pmcAlcohol dehydrogenases (ADHs EC 1.1.1.1) are NAD(P)H‐dependent medium‐chain oxidoreductases found in all kingdoms of life. These enzymes typically catalyse the reversible reduction of aldehydes or ketones to the corresponding alcohol. The structural motifs of ADHs are highly conserved in all known eukaryotic examples; most notably, a zinc ion involved in catalysis, a second zinc ion involved in maintaining protein structure, and the Rossmann peptide‐fold involved in cofactor binding. ADHs have been shown to catalyse many complex biochemical transformations in plant natural product biosynthesis, suggesting that their catalytic repertoire has been expanded.

For example, we recently reported the discovery of dihydroprecondylocarpine acetate synthase (DPAS), an ADH involved in vinblastine biosynthesis in the plant Catharanthus roseus and in ibogaine biosynthesis in the phylogenetically related species Tabernanthe iboga. The recently discovered DPAS reduces the substrate precondylocarpine acetate to yield an initial, unstable product, which is hypothesised to be dihydroprecondylocarpine acetate. The site of incorporation indicates DPAS catalyses the 1,4‐reduction of the α,β‐unsaturated iminium moiety and is thereby the first reported ADH with 1,4‐reduction activity. We report four crystal structures of apo‐ and substrate‐bound DPAS from two phylogenetically related species. These structures reveal, surprisingly, the loss of the catalytic zinc ion from the DPAS active site, indicating that zinc is not strictly required for reduction by ADHs. Although electron density for the structural zinc ion was clearly observed in all TiDPAS2 structures (the CrDPAS structure lacked electron density for this region), surprisingly, the substrate pocket lacked electron density at the expected site of the catalytic zinc. The lack of the catalytic zinc in DPAS is substantiated by the observation that two of the conserved catalytic zinc coordinating residues are mutated (His74Met and Cys168Ser). To investigate the catalytic mechanism of CrDPAS, we performed site directed mutagenesis of key residues involved in coordination of the catalytic zinc and the proton relay. A DPAS mutant in which the zinc ion coordinating residues were restored (Met74His, Ser168Cys) still reduced precondylocarpine acetate. Collectively, these findings suggest the 1,4‐α,β‐unsaturated iminium reduction catalysed by CrDPAS does not require a catalytic zinc or a proton relay, but reintroduction of these features did not abolish activity.

>[2x]MAGKSAEEEHPIKAYGWAVKDRTTGILSPFKFSRRATGDDDVRIKILYCGICHTDLASIKNEYEFLSYPLVPGMEIVGIATEVGKDVTKVKVGEKVALSAYLGCCGKCYSCVNELENYCPEVIIGYGTPYHDGTICYGGLSNETVANQSFVLRFPERLSPAGGAPLLSAGITSFSAMRNSGIDKPGLHVGVVGLGGLGHLAVKFAKAFGLKVTVISTTPSKKDDAINGLGADGFLLSRDDEQMKAAIGTLDAIIDTLAVVHPIAPLLDLLRSQGKFLLLGAPSQSLELPPIPLLSGGKSIIGSAAGNVKQTQEMLDFAAEHDITANVEIIPIEYINTAMERLDKGDVRYRFVVDIENTLTPPSEL> APPKSVIRWCTISSPEEKKCNNLRDLTQQERISLTCVQKATYLDCIKAIANNEADAISLDGGQVF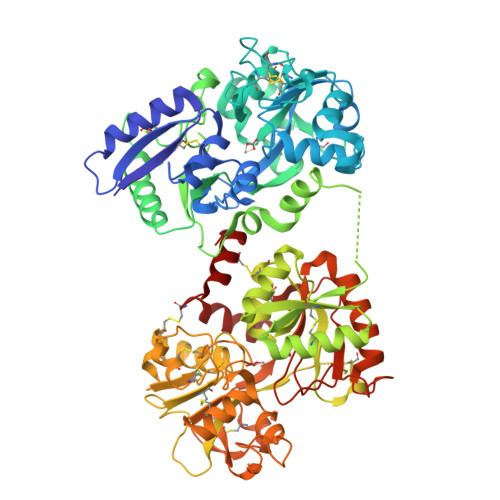EAGLAPYKLKPIAAEVYEHTEGSTTSYYAVAVVKKGTEFTVNDLQGKTSCHTGLGRSAGWNIPIGTLIHRGAIEWEGIESGSVEQAVAKFFSASCVPGATIEQKLCRQCKGDPKTKCARNAPYSGYSGAFHCLKDGKGDVAFVKHTTVNENAPDQKDEYELLCLDGSRQPVDNYKTCNWARVAAHAVVARDDNKVEDIWSFLSKAQSDFGVDTKSDFHLFGPPGKKDPVLKDLLFKDSAIMLKRVPSLMDSQLYLGFEYYSAIQSMRKDQLTPSPRENRIQWCAVGKDEKSKCDRWSVVSNGDVECTVVDETKDCIIKIMKGEADAVALDGGLVYTAGVCGLVPVMAERYDDESQCSKTDERPASYFAVAVARKDSNVNWNNLKGKKSCHTAVGRTAGWVIPMGLIHNRTGTCNFDEYFSEGCAPGSPPNSRLCQLCQGSGGIPPEKCVASSHEKYFGYTGALRCLVEKGDVAFIQHSTVEENTGGKNKADWAKNLQMDDFELLCTDGRRANVMDYRECNLAEVPTHAVVVRPEKANKIRDLLERQEKRFGVNGSEKSKFMMFESQNKDLLFKDLTKCLFKVREGTTYKEFLGDKFYTVISSLKTCNPSDILQMCSFLEGK> QFRAIIESPEGAGHVGYQYRRNTGSTMRMVSDVLDERVSLWDFHCDPSGNVIQPGPNVDSRQYLQAAIDYVSSNGGGTITIPAGYTWYLGSYGVGGIAGHSGIIQLRSNVNLNIEGRIHLSPFFDLKPFQVFVGFDNGDPASSGNLENCHIYGHGVVDFGGYEFGASSQLRNGVAFGRSYNCSVTGITFQNGDVTWAITLGWNGYGSNCYVRKCRFINLVNSSVNADHSTVYVNCPYSGVESCYFSMSSSFARNIACSVALHQHDTFYRGSTVNGYCRGAYVVMHAAEAAGAGSYAYNMQVENNIAVIYGQFVILGSDVTATVSGHLNDVIVSGNIVSIGERAAFSAPFGAFIDIGPDNSGASNVQDIQRVLVTGNSFYAPANITDSAAITLRANLNGCTFIANNFDCRYMVYNAPGTTSPVVQNLVWDKSNVIGGTHANQRAGQNLFDMQFASVVNSTIEVQLSCEDLSMFSCILFPASCQLSYSKITVDSAWTKSMSNTAVFEGNQQAGANVYVSYPATVNLTSYNTQGAVPFFSTDTNYAWVTSAYSLSINENLDFSPPATYTNKANGQLVGVGYNEIGG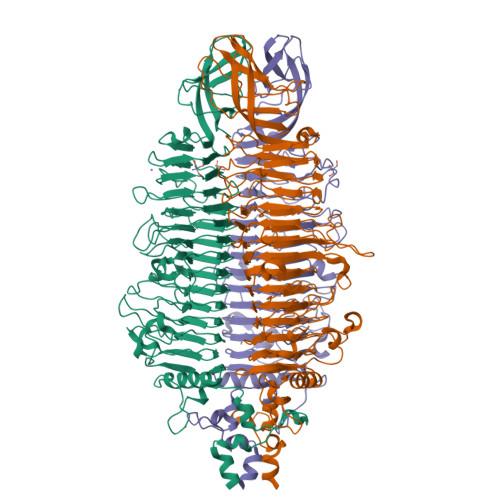VRSVSVRLMLQRQV> MSDNRRRRREEDDSDSENELPPSSPQQHFRGGMNPVSSPIGSPDMINPEGDDNEVDDVPDIDEVEEQMNEVDLMDDNMYEDYAADHNRDRYDPDQVDDREQQELSLSERRRIDAQLNERDRLLRNVAYIDDEDEEQEGAAQLDEMGLPVQRRRRRRQYEDLENSDDDLLSDMDIDPLREELTLESLSNVKANSYSEWITQPNVSRTIARELKSFLLEYTDETGRSVYGARIRTLGEMNSESLEVNYRHLAESKAILALFLAKCPEEMLKIFDLVAMEATELHYPDYARIHSEIHVRISDFPTIYSLRELRESNLSSLVRVTGVVTRRTGVFPQLKYVKFNCLKCGSILGPFFQDSNEEIRISFCTNCKSKGPFRVNGEKTVYRNYQRVTLQEAPGTVPPGRLPRHREVILLADLVDVSKPGEEVEVTGIYKNNYDGNLNAKNGFPVFATIIEANSIKRREGNTANEGEEGLDVFSWTEEEEREFRKISRDRGIIDKIISSMAPSIYGHRDIKTAVACSLFGGVPKNVNGKHSIRGDINVLLLGDPGTAKSQILKYVEKTAHRAVFATGQGASAVGLTASVRKDPITKEWTLEGGALVLADKGVCLIDEFDKMNDQDRTSIHEAMEQQSISISKAGIVTTLQARCSIIAAANPNGGRYNSTLPLAQNVSLTEPILSRFDILCVVRDLVDEEADERLATFVVDSHVRSHPENDEDREGEELKNNGESAIEQGEDEINEQLNARQRRLQRQRKKEEEISPIPQELLMKYIHYARTKIYPKLHQMDMDKVSRVYADLRRESISTGSFPITVRHLESILRIAESFAKMRLSEFVSSYDLDRAIKVVVDSFVDAQKVSVRRQLRRSFAIYTLGH;> MEGSTGFDGDATTFFAPDAVFGDRVRRFQEFLDTFTSYRDSVRSIQVYNSNNAANYNDDQDDADERDLLGDDDGDDLEKEKKAASSTSLNILPHRIIISLDDLREFDRSFWSGILVEPAYFIPPAEKALTDLADSMDDVPHPNASAVSSRHPWKLSFKGSFGAHALSPRTLTAQHLNKLVSVEGIVTKTSLVRPKLIRSVHYAAKTGRFHYRDYTDATTTLTTRIPTPAIYPTEDTEGNKLTTEYGYSTFIDHQRITVQEMPEMAPAGQLPRSIDVILDDDLVDKTKPGDRVNVVGVFKSLGAGGMNQSNSNTLIGFKTLILGNTVYPLHARSTGVAARQMLTDFDIRNINKLSKKKDIFDILSQSLAPSIYGHDHIKKAILLMLMGGVEKNLENGSHLRGDINILMVGDPSTAKSQLLRFVLNTASLAIATTGRGSSGVGLTAAVTTDRETGERRLEAGAMVLADRGVVCIDEFDKMTDVDRVAIHEVMEQQTVTIAKAGIHTTLNARCSVIAAANPVFGQYDVNRDPHQNIALPDSLLSRFDLLFVVTDDINEIRDRSISEHVLRTHRYLPPGYLEGEPVRERLNLSLAVGEDADINPEEHSNSGAGVENEGEDDEDHVFEKFNPLLQAGAKLAKNKGNYNGTEIPKLVTIPFLRKYVQYAKERVIPQLTQEAINVIVKNYTDLRNDDNTKKSPITARTLETLIRLATAHAKVRLSKTVNKVDAKVAANLLRFALLGEDIGNDIDEEESEYEEALSKRSPQKSPKKRQRVRQPASNSGSPIKSTPRRSTASSVNATPSSARRILRFQDDEQNAGEDDNDIMSPLPADEEAELQRRLQLGLRVSPRRREHLHAPEEGSSGPLTEVGTPRLPNVSSAGQDDEQQQSVISFDNVEPGTISTGRLSLISGIIARLMQTEIFEEESYPVASLFERINEELPEEEKFSAQEYLAGLKIMSDRNNLMVADDKVWRV;> MSQQSSSPTKEDNNSSSPVVPNPDSVPPQLSSPALFYSSSSSQGDIYGRNNSQNLSQGEGNIRAAIGSSPLNFPSSSQRQNSDVFQSQGRQGRIRSSASASGRSRYHSDLRSDRALPTSSSSLGRNGQNRVHMRRNDIHTSDLSSPRRIVDFDTRSGVNTLDTSSSSAPPSEASEPLRIIWGTNVSIQECTTNFRNFLMSFKYKFRKILDEREEFINNTTDEELYYIKQLNEMRELGTSNLNLDARNLLAYKQTEDLYHQLLNYPQEVISIMDQTIKDCMVSLIVDNNLDYDLDEIETKFYKVRPYNVGSCKGMRELNPNDIDKLINLKGLVLRSTPVIPDMKVAFFKCNVCDHTMAVEIDRGVIQEPARCERIDCNEPNSMSLIHNRCSFADKQVIKLQETPDFVPDGQTPHSISLCVYDELVDSCRAGDRIEVTGTFRSIPIRANSRQRVLKSLYKTYVDVVHVKVSSDKRLDVDTSTIEQELMQNKVDHNEVEEVRQITDQDLAKIREVAAREDLYSLLARSIAPSIYELEDVKKGILLQLFGGTNKTFTKGGRYRGDINILLCGDPSTSKSQILQYVHKITPRGVYTSGKGSSAVGLTAYITRDVDTKQLVLESGALVLSDGGVCCIDEFDKMSDSTRSVLHEVMEQQTISIAKAGIITTLNARSSILASANPIGSRYNPNLPVTENIDLPPPLLSRFDLVYLVLDKVDEKNDRELAKHLTNLYLEDKPEHISQDDVLPVEFLTMYISYAKEHIHPIITEAAKTELVRAYVGMRKMGDDSRSDEKRITATTRQLESMIRLAEAHAKMKLKNVVELEDVQEAVRLIRSAIKDYATDPKTGKIDMNLVQTGKSVIQRKLQEDLSREIMNVLKDQASDSMSFNELIKQINEHSQDRVESSDIQEALSRLQQEDKVIVLGEGVRRSVRL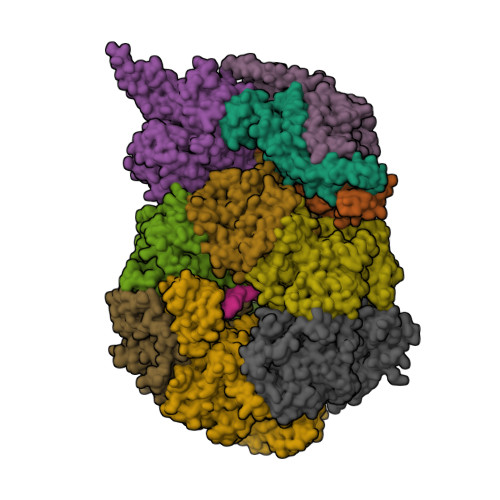NNRV;> MSFDRPEIYSAPVLQGESPNDDDNTEIIKSFKNFILEFRLDSQFIYRDQLRNNILVKNYSLTVNMEHLIGYNEDIYKKLSDEPSDIIPLFETAITQVAKRISILSRAQSANNNDKDPENTSMDTDSLLLNSLPTFQLILNSNANQIPLRDLDSEHVSKIVRLSGIIISTSVLSSRATYLSIMCRNCRHTTSITINNFNSITGNTVSLPRSCLSTIESESSMANESNIGDESTKKNCGPDPYIIIHESSKFIDQQFLKLQEIPELVPVGEMPRNLTMTCDRYLTNKVIPGTRVTIVGIYSIYNSKNGAGSGRSGGGNGGSGVAIRTPYIKILGIQSDVETSSIWNSVTMFTEEEEEEFLQLSRNPKLYEILTNSIAPSIFGNEDIKKAIVCLLMGGSKKILPDGMRLRGDINVLLLGDPGTAKSQLLKFVEKVSPIAVYTSGKGSSAAGLTASVQRDPMTREFYLEGGAMVLADGGVVCIDEFDKMRDEDRVAIHEAMEQQTISIAKAGITTVLNSRTSVLAAANPIYGRYDDLKSPGDNIDFQTTILSRFDMIFIVKDDHNEERDISIANHVINIHTGNANAMQNQQEENGSEISIEKMKRYITYCRLKCAPRLSPQAAEKLSSNFVTIRKQLLINELESTERSSIPITIRQLEAIIRITESLAKLELSPIAQERHVDEAIRLFQASTMDAASQDPIGGLNQASGTSLSEIRRFEQELKRRLPIGWSTSYQTLRREFVDTHRFSQLALDKALYALEKHETIQLRHQGQNIYRSGV;> MSSPFPADTPSSNRPSNSSPPPSSIGAGFGSSSGLDSQIGSRLHFPSSSQPHVSNSQTGPFVNDSTQFSSQRLQTDGSATNDMEGNEPARSFKSRALNHVKKVDDVTGEKVREAFEQFLEDFSVQSTDTGEVEKVYRAQIEFMKIYDLNTIYIDYQHLSMRENGALAMAISEQYYRFLPFLQKGLRRVVRKYAPELLNTSDSLKRSEGDEGQADEDEQQDDDMNGSSLPRDSGSSAAPGNGTSAMATRSITTSTSPEQTERVFQISFFNLPTVHRIRDIRSEKIGSLLSISGTVTRTSEVRPELYKASFTCDMCRAIVDNVEQSFKYTEPTFCPNPSCENRAFWTLNVTRSRFLDWQKVRIQENANEIPTGSMPRTLDVILRGDSVERAKPGDRCKFTGVEIVVPDVTQLGLPGVKPSSTLDTRGISKTTEGLNSGVTGLRSLGVRDLTYKISFLACHVISIGSNIGASSPDANSNNRETELQMAANLQANNVYQDNERDQEVFLNSLSSDEINELKEMVKDEHIYDKLVRSIAPAVFGHEAVKKGILLQMLGGVHKSTVEGIKLRGDINICVVGDPSTSKSQFLKYVVGFAPRSVYTSGKASSAAGLTAAVVRDEEGGDYTIEAGALMLADNGICCIDEFDKMDISDQVAIHEAMEQQTISIAKAGIHATLNARTSILAAANPVGGRYNRKLSLRGNLNMTAPIMSRFDLFFVILDDCNEKIDTELASHIVDLHMKRDEAIEPPFSAEQLRRYIKYARTFKPILTKEARSYLVEKYKELRKDDAQGFSRSSYRITVRQLESMIRLSEAIARANCVDEITPSFIAEAYDLLRQSIIRVDVDDVEMDEEFDNIESQSHAASGNNDDNDDGTGSGVITSEPPADIEEGQSEATARPGTSEKKKTTVTYDKYVSMMNMIVRKIAEVDREGAEELTAVDIVDWYLLQKENDLGSLAEYWEERRLAFKVIKRLVKDRILMEIHGTRHNLRDLENEENENNKTVYVIHPNCEVLDQLEPQDSS;> MSAALPSIQLPVDYNNLFNEITDFLVTFKQDTLSSDATRNENEDENLDAENIEQHLLEKGPKYMAMLQKVANRELNSVIIDLDDILQYQNEKFLQGTQADDLVSAIQQNANHFTELFCRAIDNNMPLPTKEIDYKDDVLDVILNQRRLRNERMLSDRTNEIRSENLMDTTMDPPSSMNDALREVVEDETELFPPNLTRRYFLYFKPLSQNCARRYRKKAISSKPLSVRQIKGDFLGQLITVRGIITRVSDVKPAVEVIAYTCDQCGYEVFQEVNSRTFTPLSECTSEECSQNQTKGQLFMSTRASKFSAFQECKIQELSQQVPVGHIPRSLNIHVNGTLVRSLSPGDIVDVTGIFLPAPYTGFKALKAGLLTETYLEAQFVRQHKKKFASFSLTSDVEERVMELITSGDVYNRLAKSIAPEIYGNLDVKKALLLLLVGGVDKRVGDGMKIRGDINVCLMGDPGVAKSQLLKAICKISPRGVYTTGKGSSGVGLTAAVMKDPVTDEMILEGGALVLADNGICCIDEFDKMDESDRTAIHEVMEQQTISISKAGINTTLNARTSILAAANPLYGRYNPRLSPLDNINLPAALLSRFDILFLMLDIPSRDDDEKLAEHVTYVHMHNKQPDLDFTPVEPSKMREYIAYAKTKRPVMSEAVNDYVVQAYIRLRQDSKREMDSKFSFGQATPRTLLGIIRLSQALAKLRLADMVDIDDVEEALRLVRVSKESLYQETNKSKEDESPTTKIFTIIKKMLQETGKNTLSYENIVKTVRLRGFTMLQLSNCIQEYSYLNVWHLINEGNTLKFVDDGTMDTDQEDSLVSTPKLAPQTTASANVSAQDSDIDLQDA;> MYGDLGNKLVLEAKRTKQLYARSNQDVNLPMYHEDIIRNILKEVSNLRKNTEYLKEQQQLGMLDDKVAKCQYFVTLLCMERNKRCLLAYQRLRTDILDSMAWNNNGLDLMSSITFSQQDTNNLSHQEQEYLKEYCDLITDLKSGDLVDIDLSGSLVPPSDVFIDVRVLKDAGEIQTEYGVFNLIKDSQFFVRQSDVERLIQQGYLQKI;> MSLPAHLQQTFSPEEIQFIVENEPIKIFPRITTRQKIRGDDRGTGNHTRWQLITTDDKALNNMVAMRSTEVVLWIALLLKQQSKCSIVAPQWLTTKELDRKIQYEKTHPDRFSELPWNWLVLARILFNKAKDDFHDPIHELRGKIQDLREIRQIKVLKGLKYLNESHLQLDNLSLLEINELRPFITEIMDKLREIHTASLTAGTENDEEEFNI;> MGYYDIDDVLADGTEFPCKFQYDIPGLGYLENNPGRPITKNTKLSLPLWLARILAIVGGDEALVDEEPVPFVELLPPDMFSTKVMNAIKTDPVALDLHSINSHFFSLAIKWIMLFSEKELANVVSELLLQRAQELNHHASSLSIDLNADSTGKNSANTNIATSTFLLKLEEMEKEIYKKSHESYKDTKRWMFKK;> MDINIDDILAELDKETTAVDSTKITQGSSSTTHRDANTIVGSSLDLNDKTQIYVSPQQDFSDLMKSWKNERCSPELLPYPHQLMKRLLNRISMQSQLIENISMGFLDMQNASNANPPMPNESKLPLLCMETELERLKFVIRSYIRCRLSKIDKFSLYLRQLNEDENSLISLTDLLSKDEIKYHDTHSLIWLKLVNDSILKYMPEELQAINDTEGSVNMIDEPDWNKFVFIHVNGPPDGKWNEDPLLQENEFGKPCYTVTIPDLKEEVELTIGSIYVMRYEVIRDLLRDDKVALI;> MYYGISQFSEAYNKILRNSSSHSSCQLVIFVSCLNIDALCATKMLSLLFKKQLVQSQIVPIFGYSELRRHYSQLDDNINSLLLVGFGGVIDLEAFLEIDPQEYVIDTDEKSGEQSFRRDIYVLDAHRPWNLDNIFGSQIIQCFDDGTVDDTLGEQKEAYYKLLELDEESGDDELSGDENDNNGGDDEATDADEVTDEDEEDEDETISNKRGNSSIGPNDLSKRKQRKKQIHEYEGVLEEYYSQGTTVVNSISAQIYSLLSAIGETNLSNLWLNILGTTSLDIAYAQVYNRLYPLLQDEVKRLTPSSRNSVKTPDTLTLNIQPDYYLFLLRHSSLYDSFYYSNYVNAKLSLWNENGKKRLHKMFARMGIPLSTAQETWLYMDHSIKRELGIIFDKNLDRYGLQDIIRDGFVRTLGYRGSISASEFVEALTALLEVGNSTDKDSVKINNDNNDDTDGEEEEDNSAQKLTNLRKRWVSNFWLSWDALDDRKVELLNRGIQLAQDLQRAIFNTGVAILEKKLIKHLRIYRLCVLQDGPDLDLYRNPLTLLRLGNWLIECCAESEDKQLLPMVLASIDENTDTYLVAGLTPRYPRGLDTIHTKKPILNNFSMAFQQITAETDAKVRIDNFESSIIEIRREDLSPFLEKLTLSGLL> MDHAELTTEQVLKRDIPWETYMTTK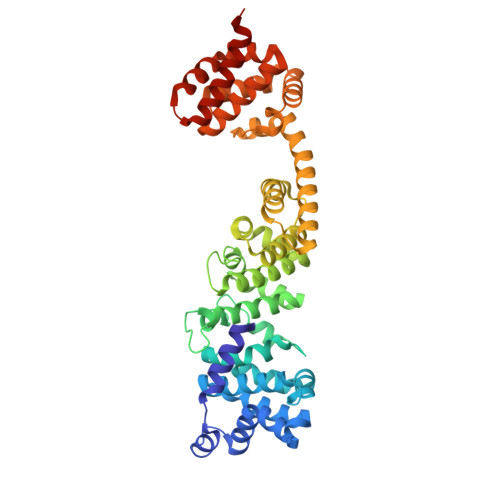LISGTGLQLLRRYDNRSESHRAQLLDDDGPSYVRVFVSILRDIYKEETVEYVLALIDEMLTANPKRARLFHDKSLASEDTYEPFLRLLWKGNWFIQEKSCKILASIVSARPKPQDRFFANGEASNSKSKSTTIDDVLKLLVEWLCAQLKKPSHPSRGVPVAINCLAALLKEPMVRSSFVQADGVKLLTPLISPASTQQSIQLLYETCLCVWLLSYYEPAVEYLATTRTLPRLIDVVKSSTKEKVVRVVVLILRNLLPKGNFAAQMIDLGLPQVVQSLKAQAWSDEDLLEGLNQLEEGLKDNIKRLSSFDKYKQEVLLGHLDWSPMHKDPLFWRDNITNFEENDFQILRVLLTILDTSSDPRALAVACFDLSQFIQYHPAGRVIVTDLKAKERVMKLMNHENTEVTKSALLCIQRLFLGAKYASFLQA>SNLSDPITGGHYENHNGYFVYIDASGKQVTGLQNIDGNLQYFDDNGYQVKGSFRDVNGKHIYFDSVTGKASSNVDIVNGKAQGYDAQGNQLKKSYVADSSGQTYYFDGNGQPLIGLQTIDGNLQYFNQQGVQIKGGFQDVNNKRIYFAPNTGNAVANTEIINGKLQGRDANGNQVKNAFSKDVAGNTFYFDANGVMLTGLQTISGKTYYLDEQGHLRKNYAGTFNNQFMYFDADTGAGKTAIEYQFDQGLVSQSNENTPHNAAKSYDKSSFENVDGYLTADTWYRPTDILKNGDTWTASTETDMRPLLMTWWPDKQTQANYLNFMSSKGLGITTTYTAATSQKTLNDAAFVIQTAIEQQISLKKSTEWLRDAIDSFVKTQANWNKQTEDEAFDGLQWLQGGFLAYQDDSHRTPNTDSGNNRKLGRQPINIDGSKDTTDGKGSEFLLANDIDNSNPIVQAEQLNWLHYLMNFGSITGNNDNANFDGIRVDAVDNVDADLLKIAGDYFKALYGTDKSDANANKHLSILEDWNGKDPQYVNQQGNAQLTMDYTVTSQFGNSLTHGANNRSNMWYFLDTGYYLNGDLNKKIVDKNRPNSGTLVNRIANSGDTKVIPNYSFVRAHDYDAQDPIRKAMIDHGIIKNMQDTFTFDQLAQGMEFYYKDQENPSGFKKYNDYNLPSAYAMLLTNKDTVPRVYYGDMYLEGGQYMEKGTIYNPVISALLKARIKYVSGGQTMATDSSGKDLKDGETDLLTSVRFGKGIMTSDQTTTQDNSQDYKNQGIGVIVGNNPDLKLNNDKTITLHMGKAHKNQLYRALVLSNDSGIDVYDSDDKAPTLRTNDNGDLIFHKTNTFVKQDGTIINYEMKGSLNALISGYLGVWVPVGASDSQDARTVATESSSSNDGSVFHSNAALDSNVIYEGFSNFQAMPTSPEQSTNVVIATKANLFKELGITSFELAPQYRSSGDTNYGGMSFLDSFL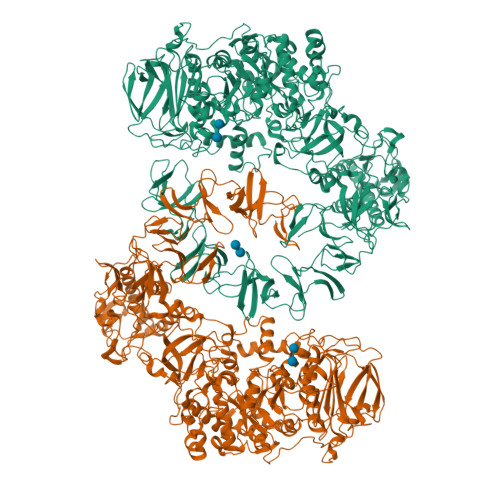NNGYAFTDRYDLGFNKADGNPNPTKYGTDQDLRNAIEALHKNGMQAIADWVPDQIYALPGKEVVTATRVDERGNQLKDTDFVNLLYVANTKSSGVDYQAKYGGEFLDKLREEYPSLFKQNQVSTGQPIDASTKIKQWSAKYMNGTNILHRGAYYVLKDWATNQYFNIAKTNEVFLPLQLQNKDAQTGFISDASGVKYYSISGYQAKDTFIEDGNGNWYYFDKDGYMVRSQQGENPIRTVETSVNTRNGNYYFMPNGVELRKGFGTDNSGNVYYFDDQGKMVRDKYINDDANNFYHLNVDGTMSR[2x]>[4x]MSQHNEKNPHQHQSPLHDSSEAKPGMDSLAPEDGSHRPAAEPTPPGAQPTAPGSLKAPDTRNEKLNSLEDVRKGSENYALTT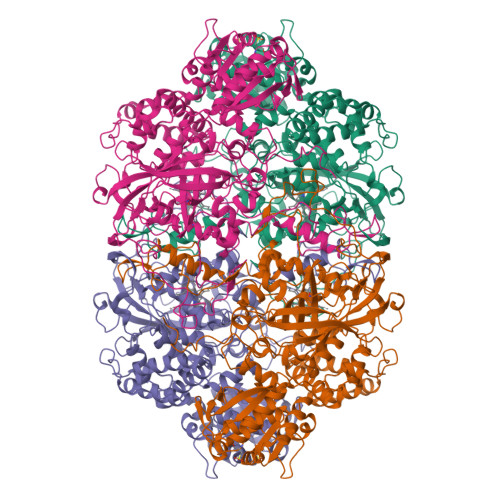NQGVRIADDQNSLRAGSRGPTLLEDFILREKITHFDHERIPERIVHARGSAAHGYFQPYKSLSDITKADFLSDPNKITPVFVRFSTVQGGAGSADTVRDIRGFATKFYTEEGIFDLVGNNTPIFFIQDAHKFPDFVHAVKPEPHWAIPQGQSAHDTFWDYVSLQPETLHNVMWAMSDRGIPRSYRTMEGFGIHTFRLINAEGKATFVRFHWKPLAGKASLVWDEAQKLTGRDPDFHRRELWEAIEAGDFPEYELGFQLIPEEDEFKFDFDLLDPTKLIPEELVPVQRVGKMVLNRNPDNFFAENEQAAFHPGHIVPGLDFTNDPLLQGRLESYTDTQISRLGGPNFHEIPINRPTCPYHNFQRDGMHRMGIDTNPANYEPNSINDNWPRETPPGPKRGGFESYQERVEGNKVRERSPSFGEYYSHPRLFWLSQTPFEQRHIVDGFSFELSKVVRPYIRERVVDQLAHIDLTLAQAVAKNLGIELTDDQLNITPPPDVNGLKKDPSLSLYAIPDGDVKGRVVAILLNDEVRSADLLAILKALKAKGVHAKLLYSRMGEVTADDGTVLPIAATFAGAPSLTVDAVIVPCGNIADIADNGDANYYLMEAYKHLKPIALAGDARKFKATIKIADQGEEGIVEADSADGSFMDELLTLMAAHRVWSRIPKIDKIPA>[4x]EKQPNIDELKKRMEQSRPNKLRGDLDQLIESDPKLRALRPHLKIDLVQEGLRIQIIDSQNRPMFKTGSAEVEPYMRDILRAIAPVLNGIPN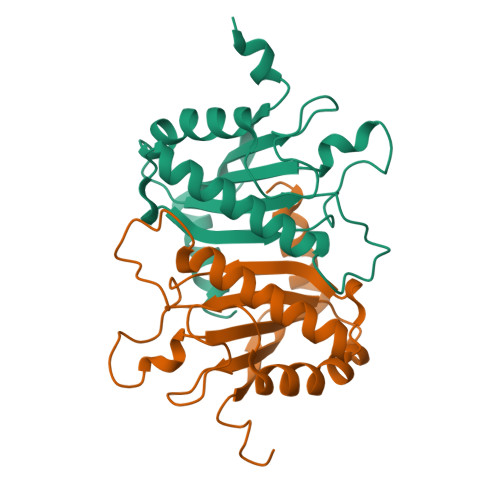RISLAGHTDDFPYANGEKGYSNWELSADRANASRRELVAGGLDNGKVLRVVGMAATMRLSDRGPDDAINRRISLLVLNKQAEQAILHHHHHH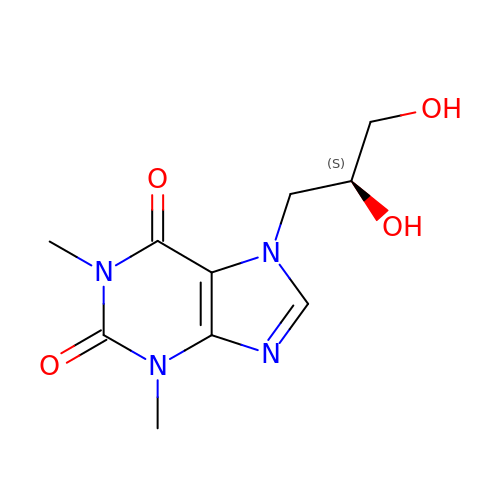7-[(2S)-2,3-DIHYDROXYPROPYL]-1,3-DIMETHYL-3,7-DIHYDRO-1H-PURINE-2,6-DIONE | C10 H14 N4 O4 | KSCFJBIXMNOVSH-LURJTMIESA-N>MGSSHHHHHHGGFSQSCLPNWIMHGKSCYLFSFSGNSWYGSKRHCSQLGAHLL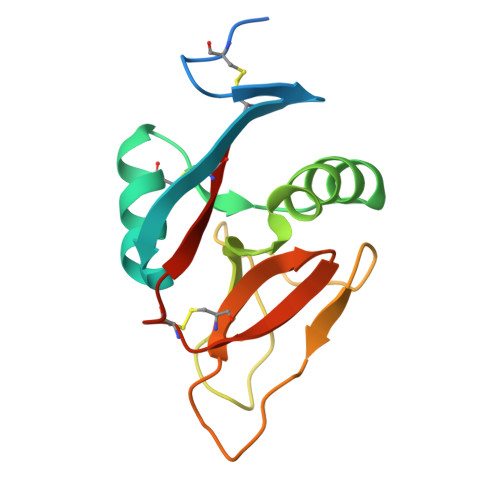KIDNSKEFEFIESQTSSHRINAFWIGLSRNQSEGPWFWEDGSAFFPNSFQVRNAVPQESLLHNCVWIHGSEVYNQICNTSSYSICEKEL[2x]> SMNPPAGPVRAIAEYERSAAVLVRYPFGIPMELIKELAKNDKVITIVASESQKNTVITQYTQSGVNLSNCDFIIAKTDSYWTRDYTGWFAMYDTNKVGLVDFIYNRPRPNDDEFPKYEAQYLGIEMFGMKLKQTGGNYMTDGYGSAVQSHIAYTENSSLSQAQVNQKMKDYLGITHHDVVQDPNGEYINHVDCWGKYLAPNKILIRKVPDNHPQHQALEDMAAYFAAQTCAWGTKYEVYRALATNEQPYTNSLILNNRVFVPVNGPASVDNDALNVYKTAMPGYEIIGVKGASGTPWLGTDALHCRTHEVADKGYLYIKHYPILGEQAGPDYKIEADVVSCANATISPVQCYYRINGSGSFKAADMTMESTGHYTYSFTGLNKNDKVEYYISAADNSGRKETYPFIGEPDPFKFTCMNETNTCTVTGAAKALRAWFNA

To this end, citrullination by the only known prokaryotic PAD expressed by keystone periodontal pathogen Porphyromonas gingivalis (PPAD) has been implicated in the aetiology of RA. PPAD is organised into four domains: the N-terminal signal peptide (NtSP, aa 1-48), catalytic/deiminase domain (CD, aa 49-360), Ig-like fold (IgLF, aa 361-463) and C-terminal domain (CTD, aa 464-556). The CD adopts the canonical fold of ββαβ motifs conserved among GME structures (RMSD 2.0–2.4 Å). The PPAD active site is an elongated cavity with its entrance exposed to the surface exterior.

Among them, a His6-tagged truncated construct (Asn49-Ala484, tPPADWT), encoding CD and IgLF but lacking NtSP and CTD, yielded highly soluble and crystallisable protein, with significantly increased catalytic activity towards the in vitro arginine substrate Nα-Benzoyl-L-arginine ethyl ester hydrochloride (BAEE) as compared with full length PPAD. We have determined the 1.46 Å and 1.48 Å structures of tPPADWT and tPPADC351A by molecular replacement, which reveal identical and superimposable conformations (root mean square deviation (RMSD)∼0.09 Å), suggesting that the Cys351Ala substitution did not perturb protein integrity. Difference Fourier electron density maps clearly reveal an active site-bound ligand, modelled in the tPPADC351A structure as an arginine-containing dipeptide, and in the tPPADWT structure as an amidino adduct where its Cζ atom is covalently linked to the Cys351 S atom. The tPPADWT structure, revealing an active site covalent adduct, captures a midway step of enzymatic turnover, likely after the Cys351 nucleophilic attack and NH3 formation steps. The acidic residues Asp238 and Asp130 serve to fixate the arginine guanidino Nη1 and Nη2 atoms by ionic interactions, thereby positioning the Cζ atom for a nucleophilic attack by the Cys351 sulphuryl group (as evidenced from the Cζ-S thioether bond in the tPPADWT structure). The imidazole group of His236 is in proximity to and at the opposite face of the guanidino plane from Cys351, and could act as a general acid/base for proton transfer. From our structural data, the arginine terminal carboxylate group is fixated by ionic interactions with Arg152 and Arg154, suggesting a role for these two basic residues in determining the reactivity of PPAD towards a C-terminal arginyl peptide substrate. As expected, tPPADWT only produced citrulline from Gly-Arg. The truncated form of PPAD secreted from P. gingivalis lacks the N-terminal 43 amino acids and CTD, and so has similar N-terminal/C-terminal boundaries to our tPPADWT construct.> GHMAKKKATETTDEDEDGGSEKKYRKCEKAGCTATCPVCFASASERCAKNGYTSRWYHLSCGEHFCNECFDHYYRSHKDGYDKYTTWKKIWTSNGKTEPSPKAFMADQQLPYWVQCTKPECRKWRQLTKEIQLTPQIAKTYRCGMKPNTAIKPETSDHCSLPEDLRVLEVSNHWWYSMLILPPLLKDSVAAPLLSAYYPDCVGMSPSCTSTNRAAATGNASPGKLEHSKAALSVHVPGMNRYFQPFYQPNECGKALCVRPDVMELDELYEFPEYSRDPTMYLALRNLILALWYTNCKEALTPQKCIPHIIVRGLVRIRCVQEVERILYFMTRKGLINTGVLSVGADQYLLPKDYHNKSVIIIGAGPAGLAAARQLHNFGIKVTVLEAKDRIGGRVWDDKSFKGVTVGRGAQIVNGCINNPVALMCEQLGISMHKFGERCDLIQEGGRITDPTIDKRMDFHFNALLDVVSEWRKDKTQLQDVPLGEKIEEIYKAFIKESGIQFSELEGQVLQFHLSNLEYACGSNLHQVSARSWDHNEFFAQFAGDHTLLTPGYSVIIEKLAEGLDIQLKSPVQCIDYSGDEVQVTTTDGTGYSAQKVLVTVPLALLQKGAIQFNPPLSEKKMKAINSLGAGIIEKIALQFPYRFWDSKVQGADFFGHVPPSASKRGLFAVFYDMDPQKKHSVLMSVIAGEAVASVRTLDDKQVLQQCMATLRELFKEQEVPDPTKYFVTRWSTDPWIQMAYSFVKTGGSG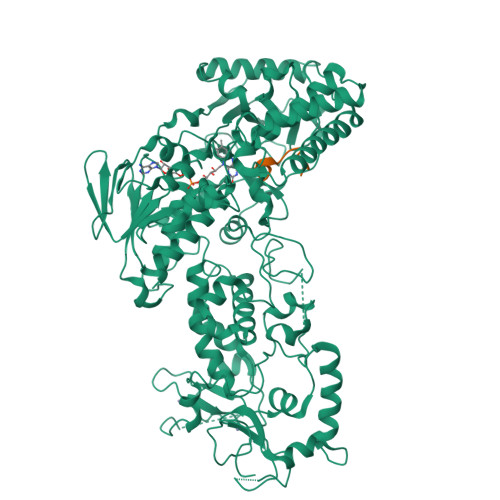EAYDIIAEDIQGTVFFAGEATNRHFPQTVTGAYLSGVREASKIAAF;> ARTMQTARKSTGGKAPRKQL1-{4-oxo-4-[(2S)-pyrrolidin-2-yl]butanoyl}-L-proline | C13 H20 N2 O4 | 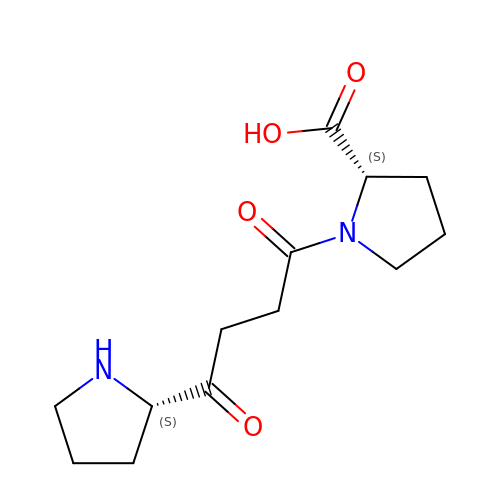FCVBOVVXXBUFFZ-UWVGGRQHSA-N>[8x]GSHMDEILARAGIFQGVEPSAIAALTKQLQPVDFPRGHTVFAEGEPGDRLYIIISGKVKIGRRAPDGRENLLTIMGPSDMFGELSIFDPGPRTSSATTITEVRAVSMDRDALRSW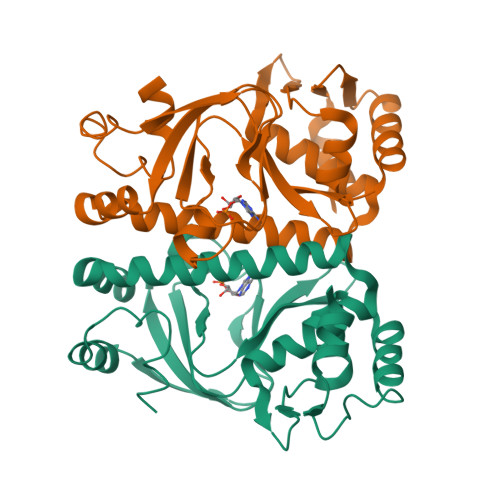IADRPEISEQLLRVLARRLRRTNNNLADLIFTDVPGRVAKQLLQLAQRFGTQEGGALRVTHDLTQEEIAQLVGASRETVNKALADFAHRGWIRLEGKSVLISDSERLARRAR>RHFEETDDAYVAGNQIQIMSQVSGSVTKVWADNTDFVKEGDVLVTLDPTDARQAFEKAKTALASSVRQTHQLMINSKQLQANIEVQKIALAKAQSDYNRRVPLGNANLIGREELQHARDAVTSAQAQLDVAIQQYNANQAMILGTKLEDQPAVQQAATEVRNAWLALERTRIISPMTGYVSRRAVQPGAQISPTTPLMAVVPATNMWVDANFKETQIANMRIGQPVTITTDIYGDDVKYTGKVVGLDMGTGSAFSLLPAQNATGNWIKVVQRLPVRIELDQKQLEQYPLRIGLSTLVSVNTTNRDGQVLANKVRSTPVAVSTAREISLAPVNKLIDDIVKANAG[6x];>ENLMQVYQQARLSNPELRKSAADRDAAFEKINEARSPLLPQLGLGADYTYSNGYRDANGINSNATSASLQLTQSIFDMSKWRALTLQEKAAGIQDVTYQTDQQTLILNTATAYFNVLNAIDVLSYTQAQKEAIYRQLDQTTQRFNVGLVAITDVQNARAQYDTVLANELTARNNLDNAVEQLRQITGNYYPELAALNVENFKTDKPQPVNALLKEAEKRNLSLLQARLSQDLAREQIRQAQDGHLPTLDLTASTGISDTSYSGSKTRGAAGTQYDDSNMGQNKVGLSFSLPIYQGGMVNSQVKQAQYNFVGASEQLESAHRSVVQTVRSSFNNINASISSINAYKQAVVSAQSSLDAMEAGYSVGTRTIVDVLDATTTLYNAKQELANARYNYLINQLNIKSALGTLNEQDLLALNNALSKPVSTNPE[3x];> AQLVIMTIALSLATFMQVLDSTIANVAIPTIAGNLGSSLSQGTWVITSFGVANAISIPLTGWLAKRVGEVKLFLWSTIAFAIASWACGVSSSLNMLIFFRVIQGIVAGPLIPLSQSLLLNNYPPAKRSIALALWSMTVIVAPICGPILGGYISDNYHWGWIFFINVPIGVAVVLMTLQTLRGRETRTERRRIDAVGLALLVIGIGSLQIMLDRGKELDWFSSQEIIILTVVAVVAICFLIVWELTDDNPIVDLSLFKSRNFTIGCLCISLAYMLYFGAIVLLPQLLQEVYGYTATWAGLASAPVGIIPVILSPIIGRFAHKLDMRRLVTFSFIMYAVCFYWRAYTFEPGMDFGASAWPQFIQGFAVACFFMPLTTITLSGLPPERLAAASSLSNFTRTLAGSIGTSITTTMWTNRESMHHAQLTESVNPFNPNAQAMYSQLEG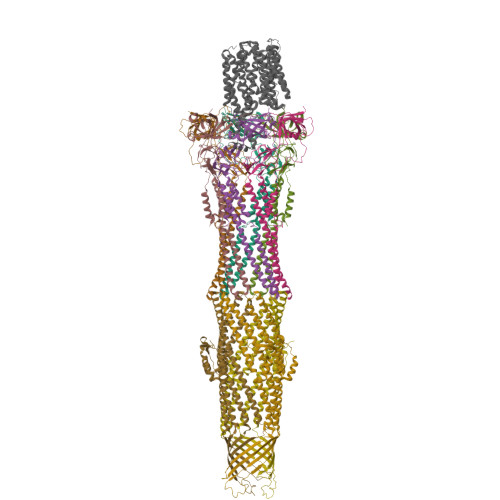LGMTQQQASGWIAQQITNQGLIISANEIFWMSAGIFLVLLGLVWFAKPPFG In this study, we identify and characterize the unique cation channel TMEM87A as a Golgi pH-regulating cation channel (GolpHCat), determine its atomic-level structure, delineate its ion conduction pathway, and ascertain its functions in Golgi homeostasis, protein glycosylation, and biological processes, and investigate its contribution to hippocampal spatial memory by employing multidisciplinary cutting-edge technologies, including Golgi-specific pH imaging, proteoliposome-single-channel recordings, cryo-EM structural analysis, molecular dynamic modeling, proteomics/glycomics approaches, and animal behavior tests. The structure of hTMEM87A contains two distinct domains: the globular domain [termed the extracellular/luminal domain (ELD), D38-K213] containing three glycans, N62, N79, and N127, and the transmembrane domain (TMD, Y224-P473) having seven transmembrane helices (7TM). Taken together, these structural analyses suggest that TMEM87A is a monomeric ion channel with a putative ion conduction pathway that can be opened by voltage stimulation and closed by PE. Taken together, these results suggest that TMEM87A might be a voltage- and pH-dependent, nonselective, and inwardly rectifying cation channel.

To address the molecular mechanism of hTMEM87A as a voltage-dependent cation channel, we determined the structure of hTMEM87A at an overall resolution of 3.1 Å using single-particle cryo-EM in the detergent condition. In the final density maps, we reliably assigned most of the side chains (D38-P473) as well as three N-linked oligosaccharides (N62, N79, and N127), except for two loops (L148–K167 and S193–L202) and the C-terminal tail (L474-E555), probably due to their structural flexibility. Based on the shape of the electron density and the lipid composition of the Golgi apparatus membrane, we modeled phosphatidylethanolamine (PE, 1-palmitoyl-2-oleoyl-sn-glycerol-3-phosphoethanolamine, or PE-16:0-18:1) to this density. Although no phospholipids had been added during protein purification, and the protein was dissolved in LMNG/CHS detergent, PE was co-purified with hTMEM87A, suggesting that PE tightly and stably binds to TMEM87A. Indeed, the lateral side of the central cavity of the TMD was partially sealed by PE, of which the R2-fatty acid chain fully occupied the lower hydrophobic cavity. In particular, the terminal amine of PE formed a charge-interaction with TM4 E347 and TM7 W445, and its phosphate group was coordinated by R305 and R309 of TM3, Y340 of TM4, and D371 of TM5. The remaining R1-fatty acid chain of PE protrudes through the gap between TM5 and TM6, where it interacts with C375, W376, and F379 of TM5 and is likely to interact with other lipid molecules in the membrane bilayer. The residues participating in these extensive interactions with PE are highly conserved, indicating a physiological role for PE in maintaining the structural and functional integrity of hTMEM87A.

> MAAAAWLQVLPVILLLLGAHPSPLSFFSAGPATVAAADRSKWHIPIPSGKNYFSFGKILFRNTTIFLKFDGEPCDLSLNITWYLKSADCYNEIYNFKAEEVELYLEKLKEKRGLSGKYQTSSKLFQNCSELFKTQTFSGDFMHRLPLLGEKQEAKENGTNLTFIGDKTAMHEPLQTWQDAPYIFIVHIGISSSKESSKENSLSNLFTMTVEVKGPYEYLTLEDYPLMIFFMVMCIVYVLFGVLWLAWSACYWRDLLRIQFWIGAVIFLGMLEKAVFYAEFQNIRYKGESVQGALILAELLSAVKRSLARTLVIIVSLGYGIVKPRLGVTLHKVVVAGALYLLFSGMEGVLRVTGAQTDLASLAFIPLAFLDTALCWWIFISLTQTMKLLKLRRNIVKLSLYRHFTNTLILAVAASIVFIIWTTMKFRIVTCQSDWRELWVDDAIWRLLFSMILFVIMVLWRPSANNQRFAFSPLSEEEEEDEQKEPMLKESFEGMKMRSTKQEPNGNSKVNKAQEDDLKWVEENVPSSVTDVALPALLDSDEERMITHFERSKME(4R,7R)-7-hydroxy-1-(4-methoxybenzyl)-7-methyl-4,5,6,7-tetrahydro-1H-benzotriazol-4-yl 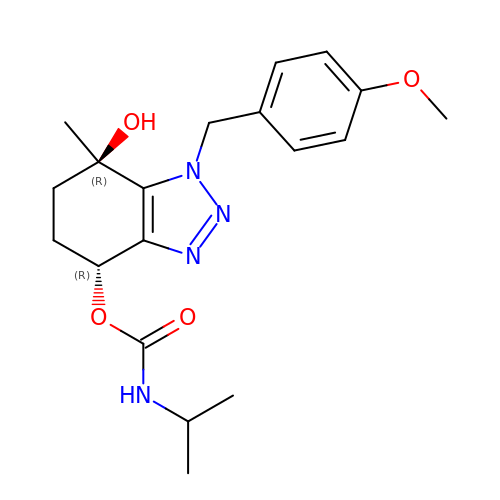propan-2-ylcarbamate | C19 H26 N4 O4 | CDAJJINZTVFCPA-DNVCBOLYSA-N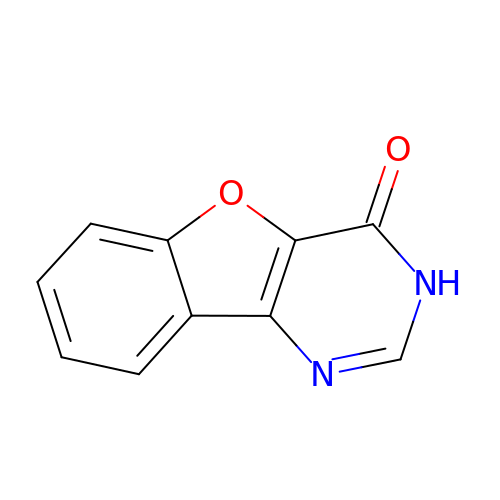BENZOFURO[3,2-D]PYRIMIDIN-4(3H)-ONE | C10 H6 N2 O2 | PCCWPSFTRGJXEF-UHFFFAOYSA-N> MDEYVQELKGLIRKHIPERCEFGHQKVTFLSQVHPSPLLTEGFKLLSSLVELESCEAHACQANTDQRFVDVILSDNGILCPTLPKVIPDGFKLTGKTLILLETFVRVNPDEFEKKWKADMSKLLNLKHDLQKSGVTLVPIVDGRSNYNNRFVADWVIERIRWLLIEILKASKSMLEIDIEDQEYQRLIHSLSNVKNQSLGLENLEHLKRNSLDYDERLNESLFIGLKGDIRESTVREELIKLKLWFKDEVFSKGLGKFKLTDRRELLESLSSLGAHLDSDVSSCPFCNNKLMEIVYNVTFSCVERTDGVATVDQQFSTTHSNIEKHYLSVLSLCNKIKGLKVFNTRRNTLLFLDLIMVNLMVDISDSCQDAIESLRKSGLIVGQMVMLVNDRVLDILEAVKLIRKKIGTNPNWVKNCSKILERSHPEIWHHLSTLIKQPDFNSLISIAQHLVSDRPIMRYSVERGSDKICRHKLFQEMSSFEQMRLFKTLSSISLSLINSMKTSFSSRLLVNEREFSKYFGNVRLRECYAQRFYLAESLVGFLFYQKTGERSRCYSVYLSDNGVMSEQGSFYCDPKRFFLPVFSDEVLAGMCEEMTSWLDFDTGLMNDTGPILRLLVLAILCSPSKRNQTFLQGLRYFLMAFANQIHHIDLTSKLVVECKSSSEVVVQRLAVGLFIRLLSGESDASLFFSRRFKYLLNVSYLCHLITKETPDRLTDQIKCFEKFIEPKVKFGCAVVNPSLNGKLTVDQEDIMINGLKKFFSKSLRDTEDVQTPGVCKELLNYCVSLFNRGKLKVSGELKNNPFRPNITSTALDLSSNKSVVIPKLDELGNILSTYDKEKLVSACVSSMAERFKTKGRYNLDPDSTDYLILKNLTGLVSAGPKAKSTQEELSLMYEALTEEQVESFNEIKHDVQVALAKMADNSVNTRTKNLGRADNSVKNGNNPLDNLWSPFGVMKEIRAEVSLHEVKDFDPDVLPPEVYKELCDAVYKSSEKCNFFLEGVLDVCPLGLLLKNLTTSSYVDEEYFMCFKYLLIQGHFDQKLGSYEHKSRSRLGFTDETLRLKDEVRLSIRESNSEAIADKLDKSYFTNAALRNLCFYSEDSPTEFTSISSNSGNLKFGLSYKEQVGSNRELYVGDLNTKLMTRLVEDFSEAVGNSMKYTCLNSEKEFERAICDMKMAVNNGDLSCSYDHSKWGPTMSPALFLALLQMLELRTPVDRSKIDLDSVKSILKWHLHKVVEVPINVAEAYCIGKLKRSLGLMGCGSTSLSEEFFHQTMQLNGQIPSHIMSVLDMGQGILHNTSDLYGLITEQFLCYALDLLYDVIPVSYTSSDDQITLIKTPSLDIEGGSDAAEWLEMICFHEFLSSKLNKFVSPKSVIGTFVAEFKSRFFVMGEETPLLTKFVAAALHNVKCKTPTQLSETIDTICDQCIANGVSTKIVTRISKRVNQLIRYSGYGETPFGAIEDQDVKDWVDGSRGYRLQRKIEAIFHDDKETSFIRNCARKVFNDIKRGRIFEENLINLIGRGGDEALTGFLQYAGCSEQEVNRVLNYRWVNLSSFGDLRLVLRTKLMTSRRVLEREEVPTLIKTLQSKLSRNFTKGVKKILAESINKSAFQSSVASGFIGFCKSMGSKCVRDGKGGFLYIKEVYSGVSACTCEICALKPKIIYCNNSLNKVSQFSKPILWDYFSLVLTNACELGEWVFSTVKEPQKPLVLNNQNFFWAVKPKVVRQIEDQLGMNHVLQSIRRNYPVLFDEHLTPFMNDLQVSRTMDSGRLKFLDVCIALDMMNENLGIISHLLKTRDNSVYIVKQSDCALAHIRQSSYTDWELGLSPQQICTNFKTQLVLSSMVNPLVLSTSCLKSFFWFNEVLELEDDSQIELAELTDFALMVKNQNVSRAMFV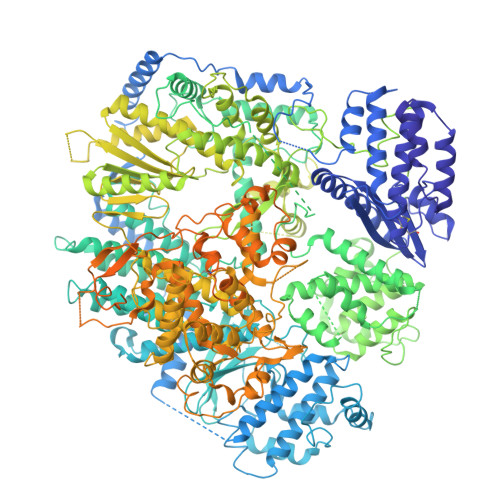EDIAMGYVVSNFEGVRISLSNVMVDGVQLPPQEKAPDIGELFGLKAENVIVGLVVQIDHVRMSTKFKLKRKMVYSFSLECIMDVGEIQNKEVILKVVAVDQSVSGSGGNHMLLDGVSVVASLPLFTGQASFDLAAMLIESNLAGSNDNFLMRNVTLDLGGFSPELSDKYSYRLSGPENQEDPLVLKDGAFYVGGERLSTYKVEFTGDLVVKALGALEDDESVVSMLHQLWPYLKATSQVILFQQEDFTIVHDLYKKQLTKSIESFGEWIEFTNFKVAYSKSLKELVISDTQGSFRLKGVMCRPLASTPQVEDIE>[4x]MKLE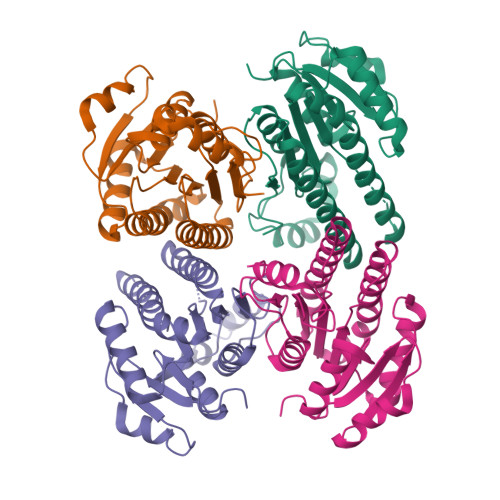HKNIFITGSSRGIGLAIAHKFAQAGANIVLNSRGAISEELLAEFSNYGIKVVPISGDVSDFADAKRMIDQAIAELGSVDVLVNNAGITQDTLMLKMTEADFEKVLKVNLTGAFNMTQSVLKPMMKAREGAIINMSSVVGLMGNIGQANYAASKAGLIGFTKSVAREVASRNIRVNVIAPGMIESDMTAILSDKIKEATLAQIPMKEFGQAEQVADLTVFLAGQDYLTGQVIAIDGGLSM1-[(2S)-2-(4-methoxyphenyl)-2,3,6,7-tetrahydro-1H-azepin-1-yl]ethan-1-one 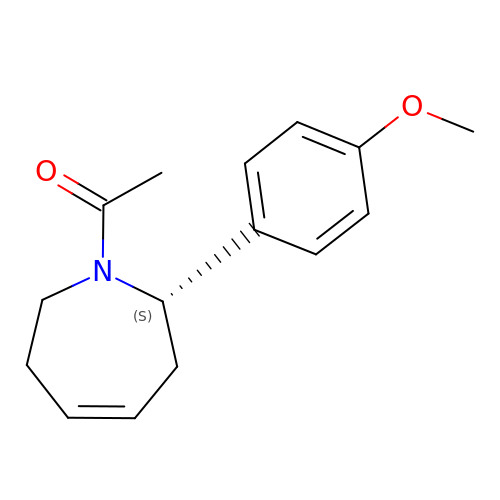| C15 H19 N O2 | GDQRKUSTNBZDEQ-HNNXBMFYSA-N>[2x]ATVISNKKAYLEKVSRDGIISALAFDQRGALKRMMASHQKEEPTTEQIVSLKRLVSEELTPYASSILLDPEYGLPAIEVKDQKAGLLLAYEKTGYD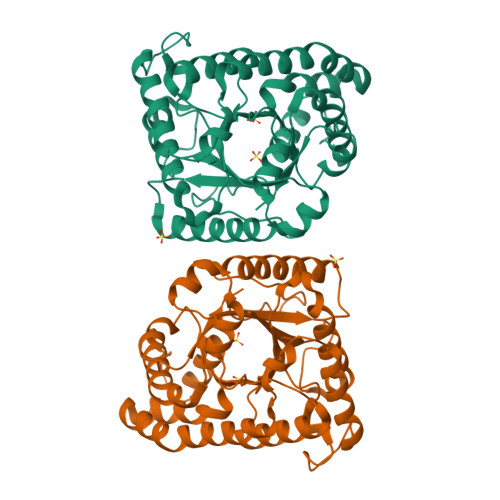AKTSSRLPDCLEDWSVKGLKAAGADAIRFLLYYDVDGNEAVNHQKKAYIERIGSECQAEDLPFFLEILTYDEKISDNSSIAFAKVKAHKVNEAMRVFSAKRFGIDVLKVEVPLNMAYVEGFTEGPILYSKADAALAFKEQEAASHLPYIYLSAGVSAQLFQETLIFAAQSGATFNGVLCGRATWADVVSVYIKEGEAAARQWLRQEGVKNIESLNDVLAKTASPWTNKVLEHHHHHH>MNTVDVNMMDNNPAARLEELRTIMKKNKIDVYILINSDEHNSEIINEKDKKIVKITNYSGADGILIVTKDKPILYVNALYELQAMNELDQNLFTLRISRIDNRDEIFETISSLEFNTIAFDGKNTSVVFYEKLRKALLNAYPKKKIVEKIIYNNNFDDVNKKDDENVLNFLVLEKSLVEIKDYPVNNKTLYIHDRKYNGACAGEKIDKLKQSLMYDIKNVDNLLLSELDEIAYLLNLRGYDYQYSPLFYSYLLFQFDREEQDFSKIVFFTTVKNLPADVKNLLEINKVIVKEYEEIVPYLRDVVIPSIPKHNDDNPDFKKYDISLSPYINLMIYKLFDRKNVLLQNSPVVKMKAVKNDVEIDNMKQAHILDGLALLQFFHWCEQKRKTKELFNETEMSLRHKVDYFRSTKKNFIFPSFSTISASGPNAAVIHYECTDKTNATIKPAIYLLDSGGQYLHGTTDVTRTTHFGEPTAEEKRIYTLVLKGHLRLRKVIFASYTNSSALDFIARENLFNNFMDYNHGTGHGVGLTLNVHEGGCSIGPVGGAPLKKNMVLSNEPGYYMKDKFGVRIENMQYVISKEITDTTEYLSFDDLTMYPYEKKLLDFSLLTNQEIKELNEYHTTIR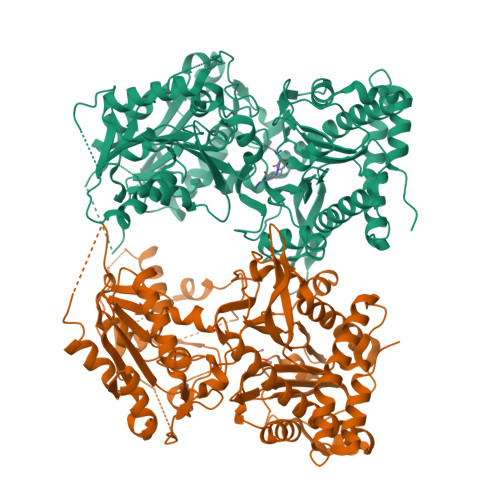NTLLPLVKQSPQEYGESVEKYLIEITEPIAIHNNHHHHHH[2x]> MGSSHHHHHHSSGLVPRGSS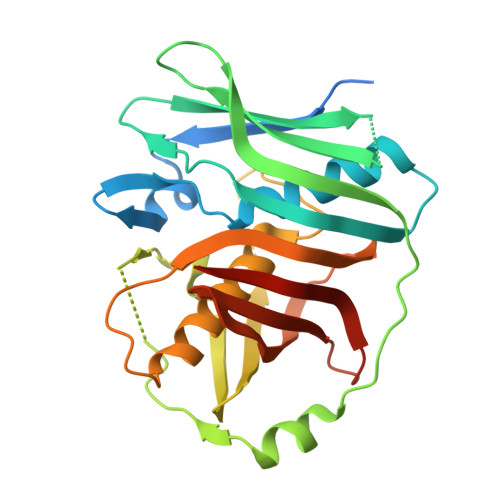DVEDNINQPVIQDQFTYDEPYVQGHVFNNERVLVGATYGSLAIEAFFNLFPEENSGRISKLSYISPIVIKQGETIELQAKPLQKDQVIELQIMYREPSSGLWKPAAIGQCGIGSFEPKKVNIENVKHSLTKLHHIDQMYKTGNGPEWGELFKTITHLYRDHKSILAKIRLPQSGLANGHHYTVSPLMTNSAYLAILSFLEQFDMTGGFLPFGINDIQFTKQTIKGDCWLLITLVKNTGDMLLFDVDVINESSETVLHYSGYSLKQLRISN> RPNGQTKPLPALKLALEYIVPCMNKHGICVVDDFLGKETGQQIGDEVRALHDTGKFTDGQLVSQKSDSSKDIRGDKITWIEGKEPGCETIGLLMSSMDDLIRHCNGKLGSYKINGRTKAMVACYPGN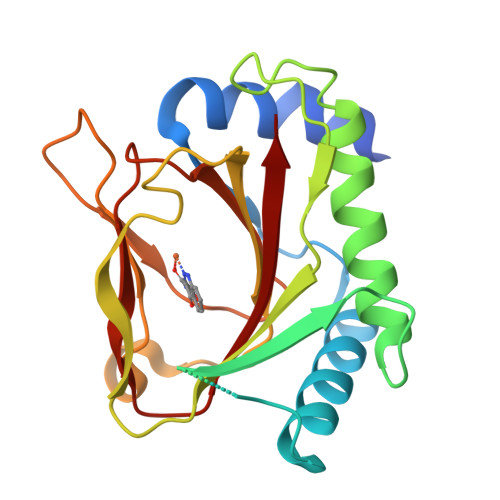GTGYVRHVDNPNGDGRCVTCIYYLNKDWDAKVSGGILRIFPEGKAQFADIEPKFDRLLFFWSDRRNPHEVQPAYATRYAITVWYFD> TIEVPVLTFVPVQVSAELENRGCWVKFFDKKNFQGDSLFLSGPATLPRLIGPFGYDWENKVRSVKVGPRANLTIFDNHNYRDEDKFLDAGANVANLSKEMGFFDN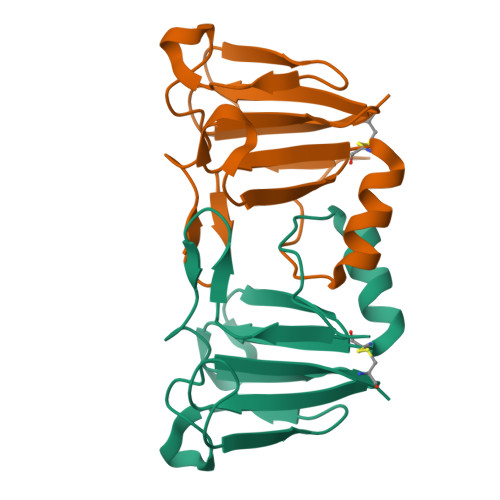FRSMVLNCI>[2x]GSHMNDVLTRVLEVVKNFEKVDASKVTPESHFVKDLGLNSLDVVE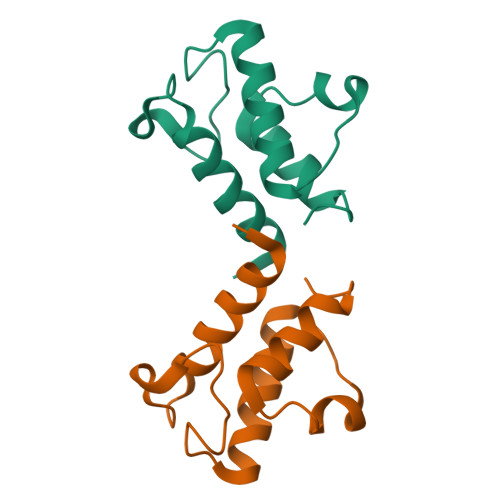VVFAIEQEFILDIPDHDAEKIQSIPDAVEYIAQNPMAK> TYVLYGIKACDTMKKARTWLDEHKVAYDFHDYKAVGIDREHLRRWCAEHGWQTVLNRAGTTFRKLDEAQKADLDEAKAIELMLAQPSMIKRPVLE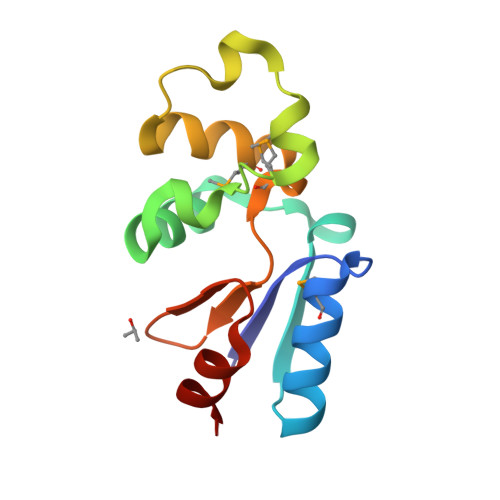LGGRTLVGFKPDAYAAALA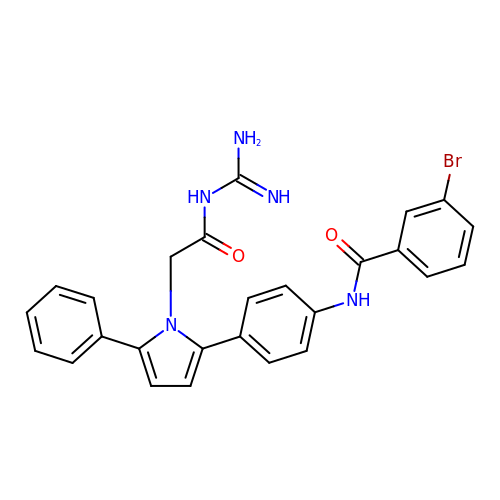3-bromo-N-[4-[1-(2-carbamimidamido-2-oxo-ethyl)-5-phenyl-pyrrol-2-yl]phenyl]benzamide | C26 H22 Br N5 O2 | XWWAMKGNSKOVNS-UHFFFAOYSA-N1-[3,5-bis(chloranyl)phenoxy]propan-2-amine 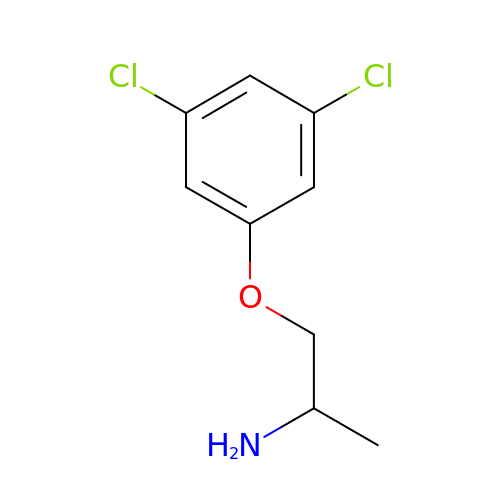| C9 H11 Cl2 N O | YNVNHWOJYTUTFH-LURJTMIESA-N>[2x]MDLPEIVASGDPVLHE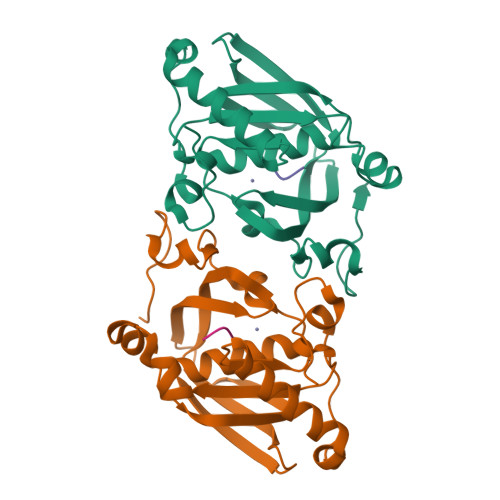KAREVDPGEIGSERIQKIIDDMIKVMRLAPGVGLAAPQIGVPLRIIVLEDTKEYISYAPKEEILAQERRHFDLMVMVNPVLKERSNKKALFFEGCLSVDGFRAAVERYLEVVVTGYDRQGKRIEVNASGWQARILQHECDHLDGNLYVDKMVPRTFRTVDNLDLPLAEGCPKLGSHHHHHH;>[2x]MAS>[2x]VIDLNASAQAMSDLDEGAINEVVDKVMAKADADAAQELIKAFQQGMTKVGERFDSGEYFIGDLIFAGEILQAAMDKLKPALSGDALEKRAKIVLATVEGDLHDIGKNIFRTMAEASGFEVFDLGIDVPVKIIVDKVKEVNPEIVGLSGVLTLALDSMRETVDALKAEGLRNDLKVIIGGVPVNENVCQRVGADDFSTNAADGVKICQRWVG

O-Demethylases belong to the class of cobalamin-dependent methyltransferases that catalyse methyl-group transfer from a methyl donor to a methyl acceptor via a methyl­cobalamin or methylcobamide acting as a reaction intermediate. In the case of the O-demethylase system, four different proteins are needed for the reaction: (i) a substrate-binding domain that serves as a methyl donor, (ii) a cobalamin-binding domain that catalyses the methyl-transfer reaction, (iii) a tetrahydrofolate-binding domain that accepts the methyl group, thus forming 5-methyltetrahydrofolate, and (iv) an activating enzyme that reduces the cobalt of cobalamin back to the catalytically active +1 state in case of occasional oxidation to the inactive +2 state. Bioinformatic studies propose that CobDH is part of a multi-component O-demethylase enzyme system.

CobDH was crystallized in the presence of methylcobalamin and the structure was refined to 1.5 Å resolution. Two CobDH monomers were found in the asymmetric unit. The overall high-resolution structure of CobDH reveals two domains that are separated by a flexible linker. The N-terminal domain (residues 1–82) folds into an antiparallel four-helix bundle. The C-terminal domain (residues 90–212) resembles a typical Rossmann fold with a central five-stranded parallel β-sheet surrounded by six α-helices that forms the binding site for the methylcobalamin. The corrin ring and the central Co atom are presented on the surface of the protein, while the dimethylbenzimidazole (DMB) base protrudes deep into the central β-sheet region. His102 forms a coordination bond towards the Co atom from the lower axial site, which results in a base-off/His-on cobalamin-binding form. No electron density has been observed at the upper axial ligand site from the Co atom. This finding leads to the conclusion that the methyl group in the crystals has been cleaved off by photoreduction during crystallization, cryoprotection or X-ray exposure, a process that has also been described for other crystal structures of methylcobalamin-dependent enzymes, resulting in the formation of cob(II)alamin. No electron density was observed corresponding to the long linker region which connects the two domains (residues 83–89), suggesting a high degree of flexibility within the linker.> ATA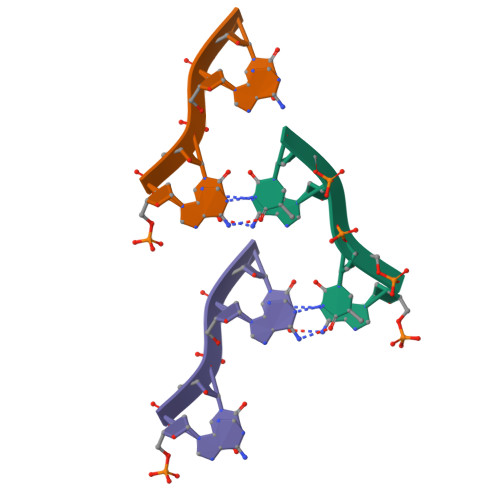T> IEIRKHLESQPVYIFTSLAGGMQVILRSNNLAAILQGNGIKFEYRDLGTDEEAKKIWKRQANGKTLPGVVRGDDYIGNWQEIE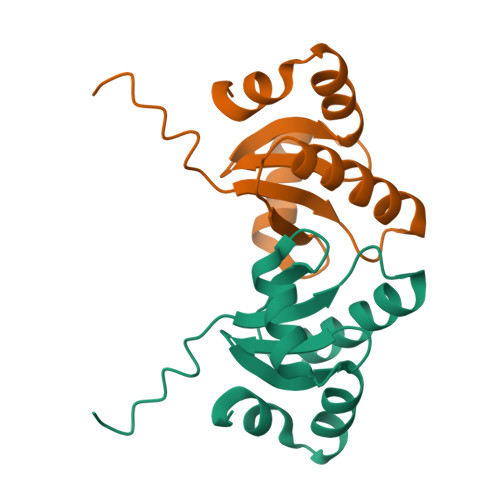DANEEYRLRELLYET>MASSINPWILTGFADAEGSFGLRIRKRNKSSVGYSTELGFEIKLHNKDKSILENIQSTWGVGVIANSGSNAVRLRVTRFEDLKVIIDHFEKYPLITQKYADYMLFKQAFNVMENKEHLTIEGIKELVRIKAKLNWGLTDELKKAFPEIISKERSLINKNIPNFKWLAGFTSGEGCFFVNLLKSKSKLGVQVCLVFSIGQHIRDKNLMNSLITYLGCGYILKKNKSEFSWLEFCVTKFSDIRDKIIPFFQEYTLIGTKLKDFEDWCKVAKLIEEK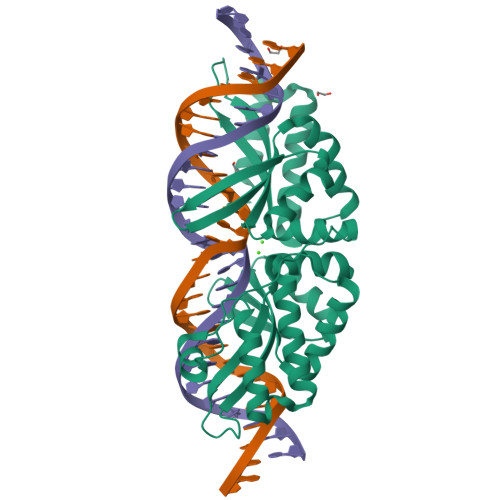KHLTEEGLDEIKKIKLNMNKGR[2x]> PISPIETVPVKLKPGMDGPKVKQWPLTEEKIKALVEICTEMEKEGKISKIGPENPYNTPVFAIKKKDSTKWRKLVDFRELNKRTQDFWEVQLGIPHPAGLKKKKSVTVLDVGDAYFSVPLDEDFRKYTAFTIPSINNETPGIRYQYNVLPQGWKGSPAIFQSSMTKILEPFKKQNPDIVIYQYMDDLYVGSDLEIGQHRTKIEELRQHLLRWGLTTPDKKHQKEPPFLWMGYELHPDKWTVQPIVLPEKDSWTVNDIQKLVGKLNWASQIYPGIKVRQLSKLLRGTKALTEVIPLTEEAELELAENREILKEPVHGVYYDPSKDLIAEIQKQGQGQWTYQIYQEPFKNLKTGKYARMRGAHTNDVKQLTEAVQKITTESIVIWGKTPKFKLPIQKETWETWWTEYWQATWIPEWEFVNTPPLVKLWYQLEKEPIVGAETFYVDGAANRETKLGKAGYVTNKGRQKVVPLTNTTNQKTELQAIYLALQDSGLEVNIVTDSQ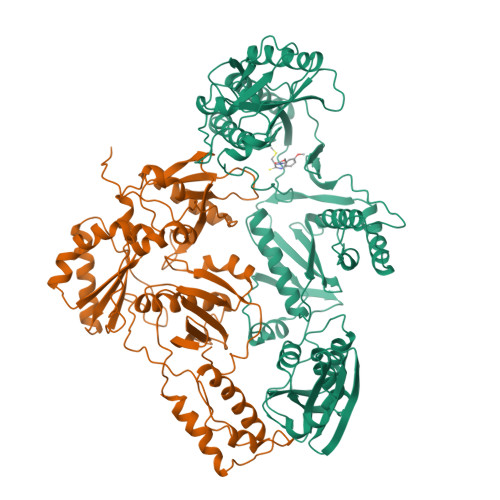YALGIIQAQPDKSESELVNQIIEQLIKKEKVYLAWVPAHKGIGGNEQVDKLVSAGI;> PISPIETVPVKLKPGMDGPKVKQWPLTEEKIKALVEICTEMEKEGKISKIGPENPYNTPVFAIKKKDSTKWRKLVDFRELNKRTQDFWEVQLGIPHPAGLKKKKSVTVLDVGDAYFSVPLDEDFRKYTAFTIPSINNETPGIRYQYNVLPQGWKGSPAIFQSSMTKILEPFKKQNPDIVIYQYMDDLYVGSDLEIGQHRTKIEELRQHLLRWGLTTPDKKHQKEPPFLWMGYELHPDKWTVQPIVLPEKDSWTVNDIQKLVGKLNWASQIYPGIKVRQLSKLLRGTKALTEVIPLTEEAELELAENREILKEPVHGVYYDPSKDLIAEIQKQGQGQWTYQIYQEPFKNLKTGKYARMRGAHTNDVKQLTEAVQKITTESIVIWGKTPKFKLPIQKETWETWWTEYWQATWIPEWEFVNTPPLVKLWYQLE> TVGAVALDLDGNLAAA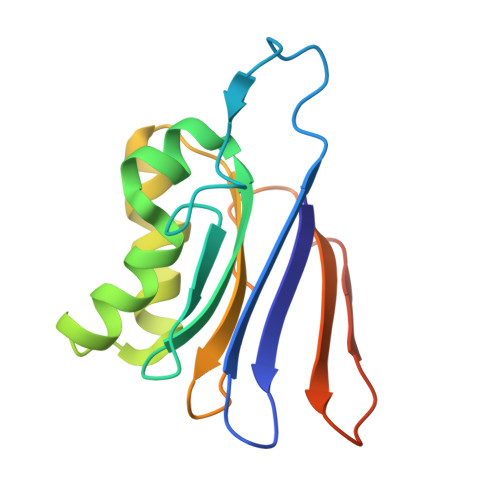TSTGGMTNKLPCSVGLVPLVGAGCYANNASVAVSCTGTGEVFIRALAAYDIAALMDYGGLSLAEACERVVMEKLPALGGSGGLIAIDHEGNVALPFNTEGMYRAWGYAGDTPTTGIYREKGDTVATQ>[2x]MSALFEPYTLKDVTLRNRIAIPPMCQYMAEDGLINDWHQVHYASMARGGAGLLVVEATAVAPEGRITPGCAGIWSDAHAQAFVPVVQAIKAAGSVPGIQIAHAGRKASANRPWEGDDHIGADDARGWETIAPSAIAFGAHLPNVPRAMTLDDIARVKQDFVDAARRARDAGFEWIELHFAHGYLGQSFFSEHSNKR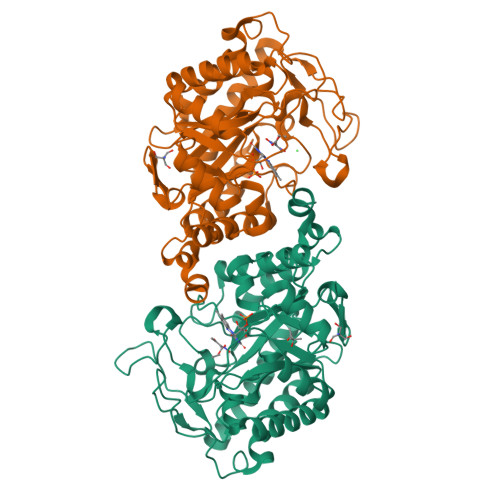TDAYGGSFDNRSRFLLETLAAVREVWPENLPLTARFGVLEYDGRDEQTLEESIELARRFKAGGLDLLSVSVGFTIPETNIPWGPAFMGPIAERVRREAKLPVTSAWGFGTPQLAEAALQANQLDLVSVGRAHLADPHWAYFAAKELGVEKASWTLPAPYAHWLERYRRPHHHHHH>[2x]GGGRMDAATTRVGLTDLTFRLLRESFADAVSWVAKNLPARPAVPVLSGVLLTGSDNGLTISGFDYEVSAEAQVGAE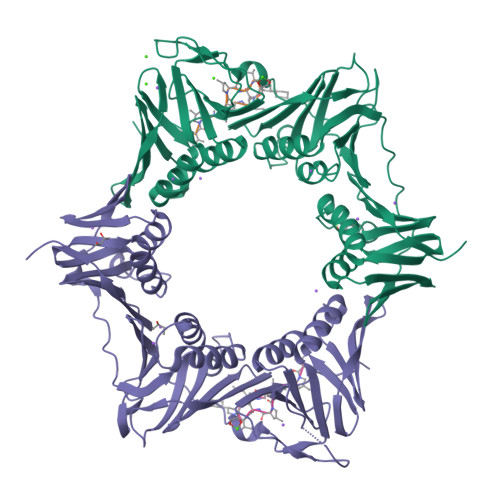IVSPGSVLVSGRLLSDITRALPNKPVDVHVEGNRVALTCGNARFSLPTMPVEDYPTLPTLPEETGLLPAELFAEAISQVAIAAGRDDTLPMLTGIRVEILGETVVLAATDRFRLAVRELKWSASSPDIEAAVLVPAKTLAEAAKAGIGGSDVRLSLGTGPGVGKDGLLGISGNGKRSTTRLLDAEFPKFRQLLPTEHTAVATMDVAELIEAIKLVALVADRGAQVRMEFADGSVRLSAGADDVGRAEEDLVVDYAGEPLTIAFNPTYLTDGLSSLRSERVSFGFTTAGKPALLRPVSGDDRPVAGLNGNGPFPAVSTDYVYLLMPVRLPG;>XVPTLPLVPXG[2x]> HTSPLLAPVRQIHAFGDSYSDNGESQRLTREMLAKGIAGAQALPGEVYWQGRWSNGPTAVEVLARQLGAQLADHAVGGAKSGADNYYGWMSAYRHTGLAGQVDAYLATLDGKPVDGQALHFIFVSANDFFEHEDFAGEQPLEQLAGSSVANIRAAVQ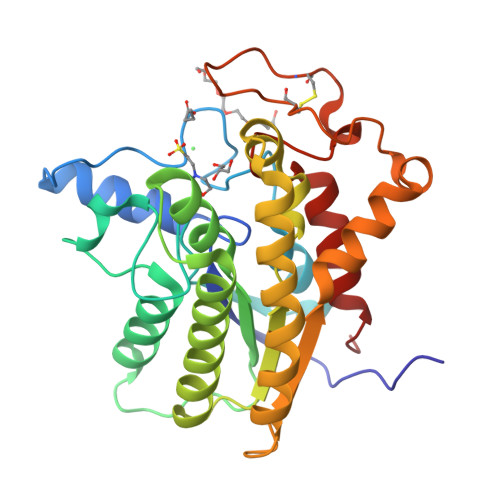RLGEAGARRFLVVSSTDLSVVPAVVAGNRVERAQRYLQAVNASLPIQLAALRKTRGLELSWFDHLTFSRHLRRNPARYGLVELDAPCQPTQPSVRPACANPDQYYFWDEWHPTRRVHQLAGEAMAARYAR>ERSAVQLSLSSRLQLTLYQYKTCPFCSKVRAFLDFHALPYQVVEVNPVLRAEIKFSSYRKVPILVAQEGESSQQLNDSSVIISALKTYLVSGQPLEEIITYYPAMKAVNDQGKEVTEFGNKYWLMLNEKEAQQVYSGKEARTEEMKWRQWADDWLVHLISPNVYRTPTEALASFDYIVREGKFGAVEGAVAKYMGAAAMYLISKRLKSRHRLQDNVREDLYEAADKWVAAVGKDRPFMGGQKPNLADLAVYGVLRVMEGLDAFDDLMQHTHIQPWYLRVERAITEA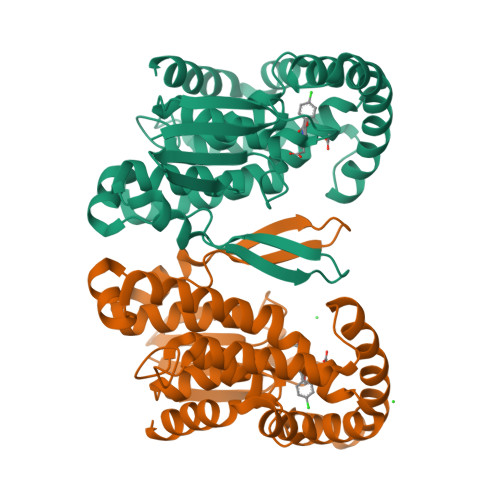SPAH[4x]> MRGSHHHHHHTDQFTMEQNPQSQLKLLVTRGKEQGYLTYAEVNDHLPEDIVDSDQIEDIIQMINDMGIQVMEEAPDADDLMLAENTADEDAAEAAAQVLSSVESEIGRTTDPVRMYMREMGTVELLTREGEIDIAKRIEDGINQVQCSVAEYPEAITYLLEQYDRVEAEEARLSDLITGFVDPNAEEDLAPTATHVGSELSQEDLDDDEDEDEEDGDDDSADDDNSIDPELAREKFAELRAQYVVTRDTIKAKGRSHATAQEEILKLSEVFKQFRLVPKQFDYLVNSMRVMMDRVRTQERLIMKLCVEQCKMPKKNFITLFTGNETSDTWFNAAIAMNKPWSEKLHDVSEEVHRALQKLQQIEEETGLTIEQVKDINR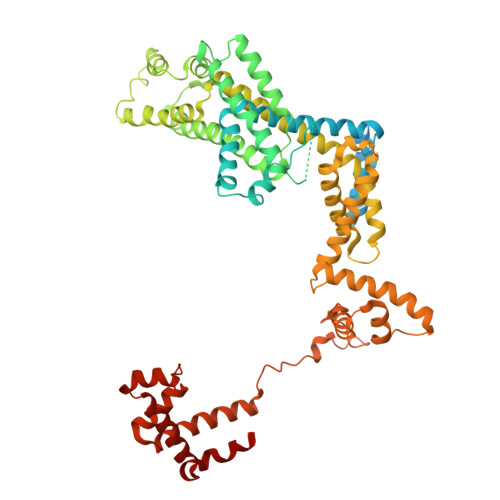RMSIGEAKARRAKKEMVEANLRLVISIAKKYTNRGLQFLDLIQEGNIGLMKAVDKFEYRRGYKFSTYATWWIRQAITRSIADQARTIRIPVHMIETINKLNRISRQMLQEMGREPTPEELAERMLMPEDKIRKVLKIAKEPISMETPIGDDEDSHLGDFIEDTTLELPLDSATTESLRAATHDVLAGLTAREAKVLRMRFGIDMNTDYTLEEVGKQFDVTRERIRQIEAKALRKLRHPSRSEVLRSFLDD>[2x]MGSLVCVGTGLQLAGQISVLSRSYIEHADIVFSLLPDGFSQRWLT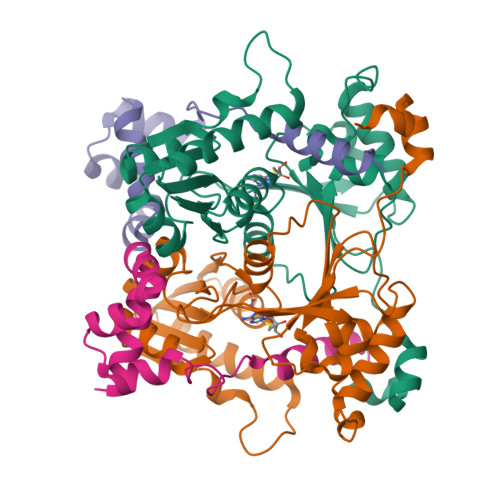KLNPNVINLQQFYAQNGEVKNARDTYEQMVNAILDAVRAGKKTVCALYGHPGVFACVSHMAITRAKAEGFSAKMEPGISAEACLWADLGIDPGNSGHQSFEASQFMFFNHVPDPTTHLLLWQIAIAGEHTLTQFHTSSDRLQILVEQLNQWYPLDHEVVIYEAANLPIQAPRIERLPLANLPQAHLMPISTLLIPPAKKLEYNYAILAKLGIGPEDLG;>[2x]HHMSGLSDFFTQLGQDAQLMEDYKQNPEAVMRAHGLTDEQINAVMTGDMEKLKTLSGDSSYQSYLVISHGNGD> SPIMNLEQSPLEEDMSLFGDVFSEQDGVDFNTLLQSMKDEFLKTLNLSDIPTQDSAKVDPPEYMLELYNKFATDRTSMPSANIIRSFKNEDLFSQPVSFNGLRKYPLLFNVSIPHHEEVIMA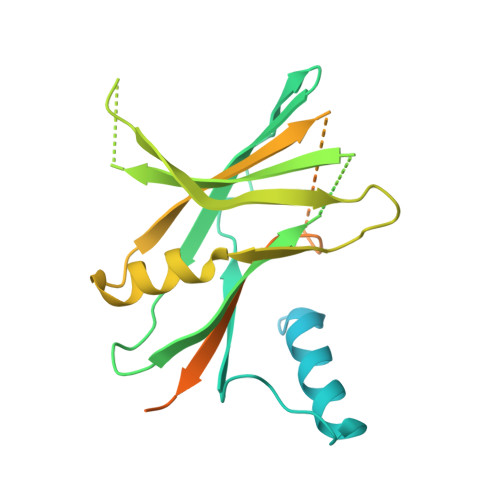ELRLYTLVQRDRMIYDGVDRKITIFEVLESKGDNEGERNMLVLVSGEIYGTNSEWETFDVTDAIRRWQKSGSSTHQLEVHIESKHDEAEDASSGRLEIDTSAQNKHNPLLIVFSDDQSSDKERKEELNEMISHEQLPELDNLGLDSFSSGPGEEALLQMRSNIIYDSTARIRR>[8x]GSMPGFLTAFEYSEKRKMVFHITTGSQEFDKLLGGGIESMAITEAFGEFRTGKTQLSHTLCVTAQLPGAGGYPGGKIIFIDTENTFRPDRLRDIADRFNVDHDAVLDNVLYARAYTSEHQMELLDYVAAKFHEEAGIFKLLIIDSIMALFRVDFSGRGELAERQQKLAQMLSRLQKISEEYNVAVFVTNQMTADPGATMTFQADPKKPIGGHILAHASTTRISLRKGRGELRIAKI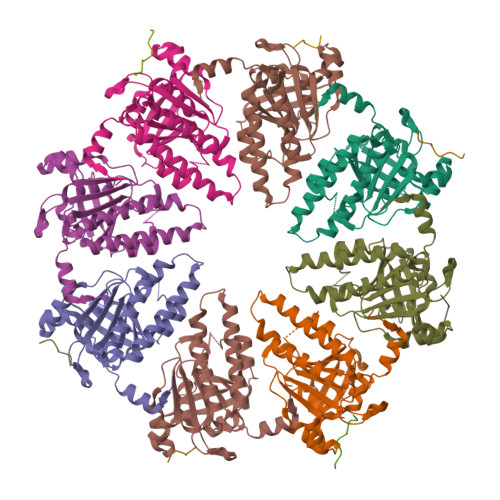YDSPEMPENEATFAITAGGIGDAKE;>GRPTKVFVPPFKTK[7x]>GGMAERSLLTGEEGWRTYKATGPRLSLPRLVALLKGQGLEVGKVAEAEGGFYVDLRPEARPEVAGLRLEPA[2x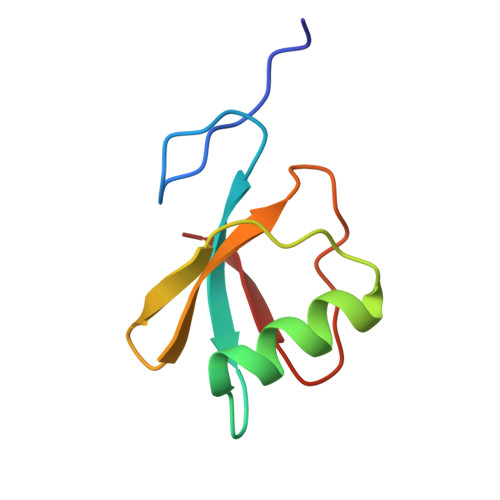]> MANVPWAEVCEKFQAALALSRVELHKNPEKEPYKSKYSARALLEEVKALLGPAPEDEDERPEAEDGPGAGDHALGLPAEVVEPEGPVAQRAVRLA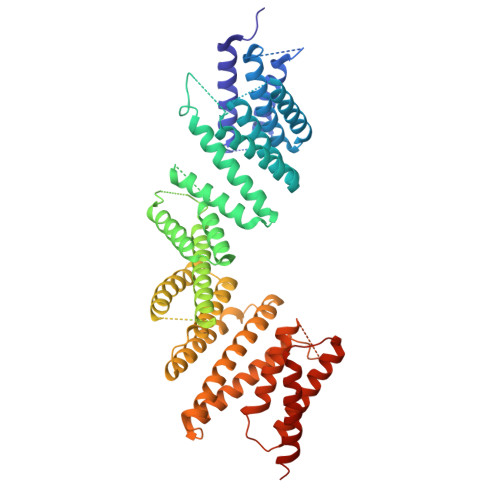VIEFHLGVNHIDTEELSAGEEHLVKCLRLLRRYRLSHDCISLCIQAQNNLGILWSEREEIETAQAYLESSEALYNQYMKEVGSPPLDPTERFLPEEEKLTEQERSKRFEKVYTHNLYYLAQVYQHLEMFEKAAHYCHSTLKRQLEHNAYHPIEWAINAATLSQFYINKLCFMEARHCLSAANVIFGQTGKISATEDTPEAEGEVPELYHQRKGEIARCWIKYCLTLMQNAQLSMQDNIGELDLDKQSELRALRKKELDEEESIRKKAVQFGTGELCDAISAVEEKVSYLRPLDFEEARELFLLGQHYVFEAKEFFQIDGYVTDHIEVVQDHSALFKVLAFFETDMERRCKMHKRRIAMLEPLTVDLNPQYYLLVNRQIQFEIAHAYYDMMDLKVAIADRLRDPDSHIVKKINNLNKSALKYYQLFLDSLRDPNKVFPEHIGEDVLRPAMLAKFRVARLYGKIITADPKKELENLATSLEHYKFIVDYCEKHPEAAQEIEVELELSKEMVSLLPTKMERFRTKMALT> ETGKETAFVEVVLFESS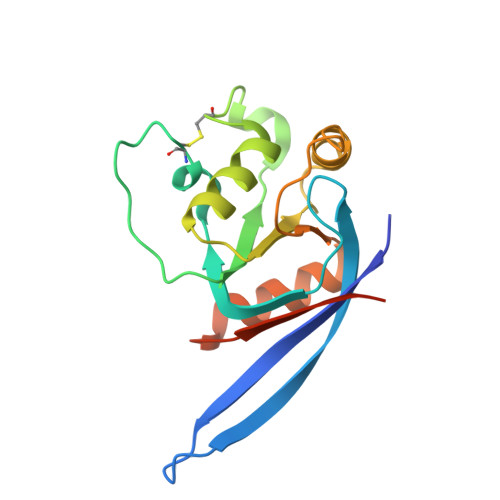PSGDYTTHTTGLTGRFSRAGAMLSAEGEIVQMHPLGLCNNNDEEDLYEYGWVGVVKLEQPELDPKPCLTVLGKAKRAVQRGATAVIFDVSENPEAIDQLNQGSEDPLKRPVVYVKGADAIKLMNIVNKQKVARARIQHLGTKHHHHHH>[2x]QDKAVDLFLDMLKEDTGTVEAHLTLGNLFRSRGEVDRAIRIHQTLMESASLTYEQRLLAIQQLGRDYMAAGLYDRAEDMFNQLTDETDFRIGALQQLLQIYQATSEWQKAIDVAERLVKLGKDKQRVEIAHFYCELALQHMA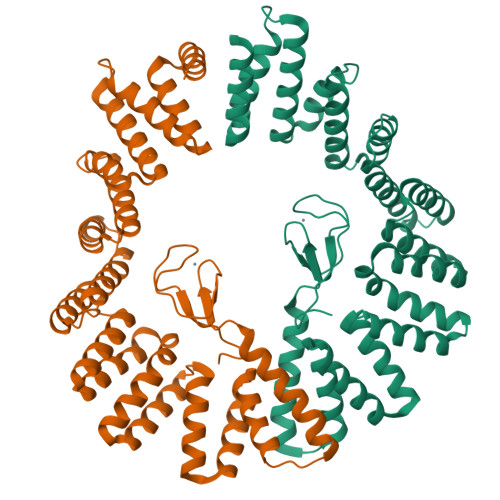SDDLDRAMTLLKKGAAADKNSARVSIMMGRVFMAKGEYAKAVESLQRVISQDRELVSETLEMLQTCYQQLGKTAEWAEFLQRAVEENTGADAELMLADIIEARDGSEAAQVYITRQLQRHPTMRVFHKLMDYHLNEAEEGRAKESLMVLRDMVGEKVRSKPRYRCQKCGFTAYTLYWHCPSCRAWSTIKPIRGLDGL[(1~{R})-1-[2-[[2,5-bis(chloranyl)phenyl]carbonylamino]ethanoylamino]-3-methyl-butyl]boronic 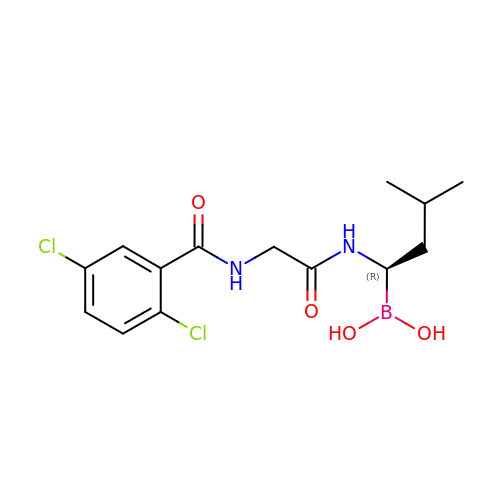acid | C14 H19 B Cl2 N2 O4 | MXAYKZJJDUDWDS-LBPRGKRZSA-N>MVLYFIGLGLYDERDITVKGLMIAKKCDYVFAEFYTSLMAGTTLGRIQKLIGKEIRVLSREDVELNFENIVLPLAKENDVAFLTPGDPLVATTHAELRIRAK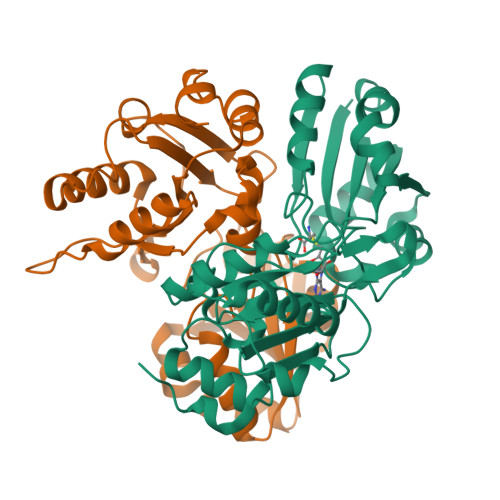RAGVESYVIHAPSIYSAVGITGLHIYKFGKSATVAYPEGNWFPTSYYDVIKENAERGLHTLLFLDIKAEKRMYMTANEAMELLLKVEDMKKGGVFTDDTLVVVLARAGSLNPTIRAGYVKDLIREDFGDPPHILIVPGKLHIVEAEYLVEIAGAPREILRVNV[2x]> GAMDSSSRQYREKLKQVEEYMQYRKLPSHLRNKILDYYEYRYRGKMFDERHIFREVSESIRQDVANYNCRDLVASVPFFVGADSNFVTRVVTLLEFEVFQPADYVIQEGTFGDRMFFIQQGIVDIIMSDGVIATSLSDGSYFGEICLLTRERRV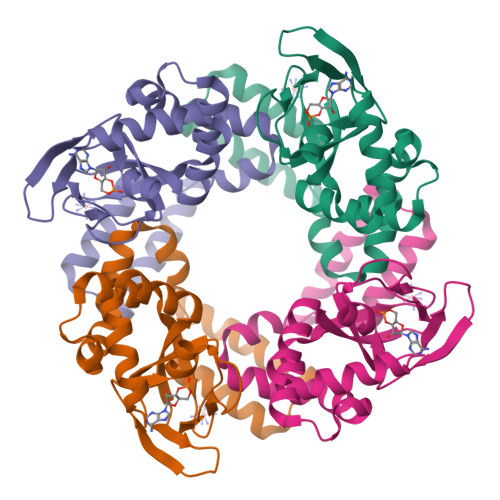ASVKCETYCTLFSLSVQHFNQVLDEFPAMRKTMEEIAVRRLTRI> MKKGHHHHHHENLYFQGGSRKKIFKPEELRQALMPTLEALYRQDPESLPFR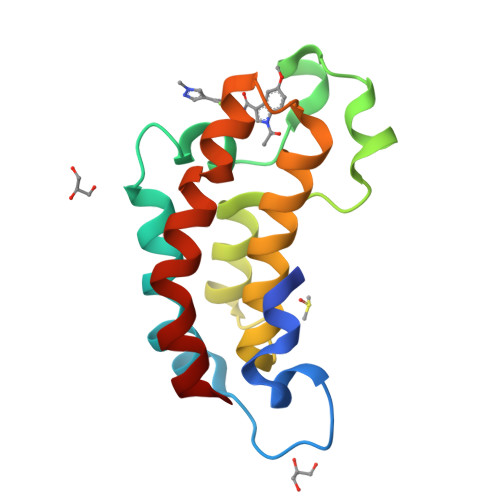QPVDPQLLGIPDYFDIVKNPMDLSTIKRKLDTGQYQEPWQYVDDVWLMFNNAWLYNRKTSRVYKFCSKLAEVFEQEIDPVMQSLG3-HYDROXYISOXAZOLE-4-CARBOXYLIC ACID | C4 H3 N O4 | 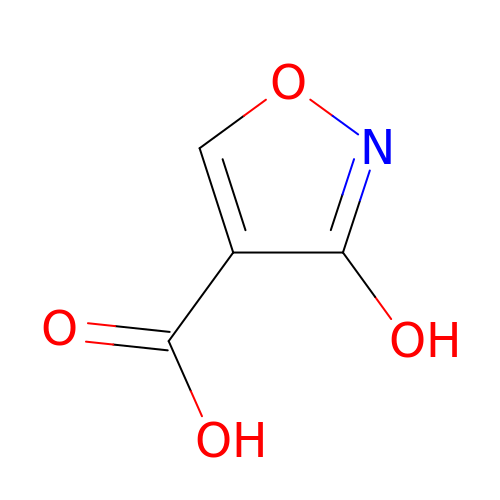JLPHBZYAQYOJND-UHFFFAOYSA-N Ionotropic glutamate receptors (iGluRs) mediate the majority of fast excitatory neurotransmission at the chemical synapses in the central nervous system (CNS). AMPA, KA, and NMDA receptors form tetrameric cation conductive channels that are activated by presynaptically released glutamate resulting in an influx of sodium and calcium ions leading to membrane depolarization. KA receptors are abundantly expressed in hippocampus and cerebellum; display characteristic slow kinetics, are mainly involved in long-term memory formation and motor control. They are divided into two families consisting of the “low-affinity” glutamate binding subunits (GluK1-GluK3) that form functional homomeric ion channels and “high-affinity” subunits (GluK4 and GluK5) that form functional receptors only on assembly with “low-affinity” subunits. In order to understand the conformational changes underlying GluK3 functions in the context of full-length tetrameric receptors and to explore the role of N-glycans in modulating their functions, we expressed and purified rat GluK3 receptors from baculovirus-infected HEK293 GnTI− cells; trapped them in agonist and antagonist bound states and determined their structures via single particle cryo-electron microscopy.

We also solved crystal structure of GluK3 ligand binding domain in complex with agonist SYM. Interestingly, GluK3 residue D759 from one protomer faces D730 from other protomer on LBD dimer formation. This close apposition of two similarly charged residues likely destabilizes the dimer interface by electrostatic repulsion. Binding of Zn ion at this site is shown to increase the dimer stability and potentiate GluK3 currents.

>GSNRSLIVTTLLEEPFVMFRKSDRTLYGNDRFEGYCIDLLKELAHILGFSYEIRLVEDGKYGAQDDKGQWNGMVKELIDHKADLAVAPLTITHVREKAIDFSKPFMTLGVSILYRKGTPIDSADDLAKQTKIEYGAVKDGATMTFFKKSKISTFEKMWAFMSSKPSALVKNNEEGIQRTLTADYALLMESTTIEYITQRNCNLTQIGGLIDSKGYGIGTPMGSPYRDKITIAILQLQEEDKLHIMKEKWWRGSGCPE[2x]>[4x]MNSTPKGTIYLTFDDGPVNASVEVIKVLNQGGVKATFYFNAWHLDGIGDENEDRALEALKLALDSGHIVGNHSYDHMIHNCVEEFGPTSGADCNATGNHQIHSYQDPVRDAASF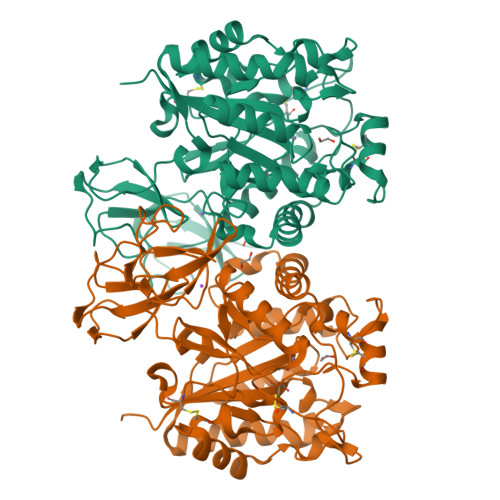EQNLITLEKYLPTIRSYPNYKGYELARLPYTNGWRVTKHFQADGLCATSDNLKPWEPGYVCDPANPSNSVKASIQVQNILANQGYQTHGWDVDWAPENWGIPMPANSLTEAVPFLAYVDKALNSCSPTTIEPINSKTQEFPCGTPLHADKVIVLTHDFLFEDGKRGMGATQNLPKLAEFIRIAKEAGYVFDTMDNYTPRWSVGKTYQAGEYVLYQGVVYKAVISHTAQQDWAPSSTSSLWTNADPATNWTLNVSYEQGDIVNYKGKRYLVSVPHVSQQDWTPDTQNTLFTALELRRQWSHPQFEK>WTTRGFVFTRHSQTTAIPSCPEGTVPLYSGFSFLFVQGNQRAHGQDLGTLGSCLQRFTTMPFLFCNVNDVCNFASRNDYSYWLSTPALMPMNMAPITGRALEPYISRCTVCEGPAIAIAVHSQTTDIPPCPHGWISLWKGFSFIMFTSAGSEGTGQALASPGSCLEEFRASPFLECHGRGTCNYYSNSYSFWLASLNPERMFRKPIPSTVKAGELEKIISRCQVCMK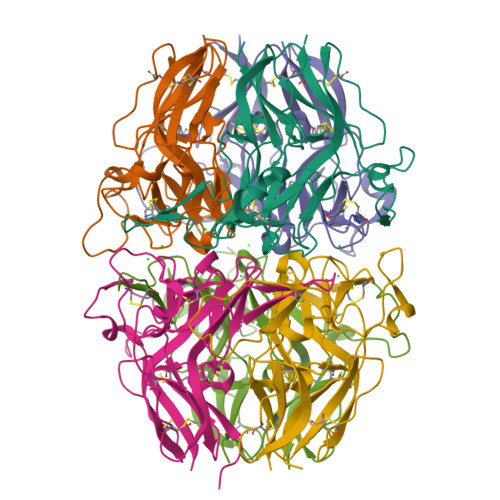KRH[8x]>GSDRPTPVPLPNSEQFYLENDRGEPYLIQVSWPLHWEDKQTGRGPLPIIYIVDGNALFLTATEAAWRRAAASHFAGGGIIVAIGYPLKGKLYDARRRSFDLTPPTACAPVGYGGADVFLDFIENSVRPAVQARFPQVSLAREALYGHSYGGLLALHALFTRPQSFDCYIASSPS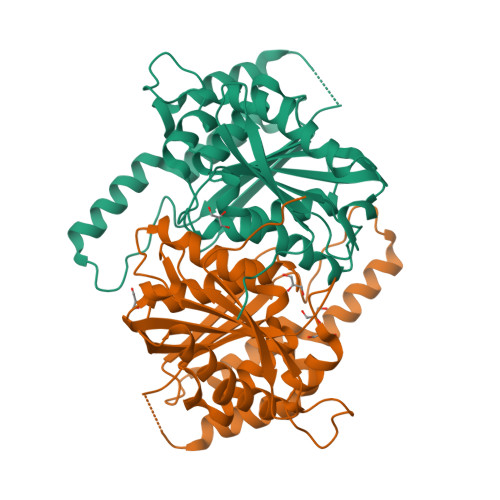IWWNSLCILHEAKAFVETKKVSHDQSPSLMVSWGSWEQHPPRWADELLDHYEARKRTAAELRMADNALDLCAMLHGCSRLHALIKTEYEGEDNTSVMSCSVSRGLTMFFEDWPFHQSG[2x]> MQTLHALLRDIPAPDAEAMARTQQHIDGLLKPPGSLGRLETLAVQLAGMPGLNGTPQVGEKAVLVMCADHGVWDEGVAVSPKIVTAIQAANMTRGTTGVCVLAAQAGAKVHVIDVGIDAEPIPGVVNMRVARGCGNIAVGPAMSRLQAEALLLEVSRYTCDLAQRGVTLFGVG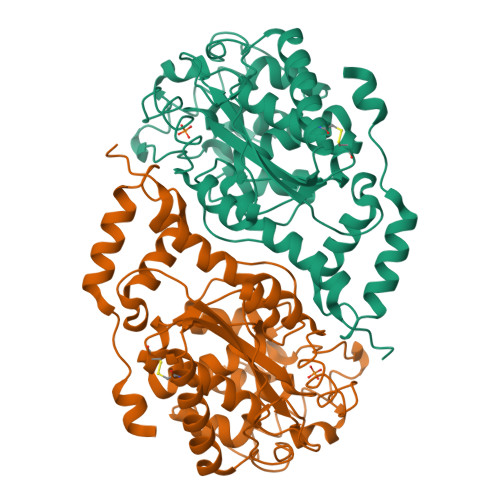ELGMANTTPAAAMVSVFTGSDAKEVVGIGANLPPSRIDNKVDVVRRAIAINQPNPRDGIDVLSKVGGFDLVGMTGVMLGAARCGLPVLLDGFLSYSAALAACQIAPAVRPYLIPSHFSAEKGARIALAHLSMEPYLHMAMRLGEGSGAALAMPIVEAACAMFHNMGELAASNIVLPEGNANAT> MLNQELELSLNMAFARAREHRHEFMTVEHLLLALLSNPSAREALEACSVDLVALRQELEAFIEQTTPVLPASEEERDTQPTLSFQRVLQRAVFHVQSSGRNEVTGANVLVAIFSEQESQAAYLLRKHEVSRLDVVNFISHGTRKDEPTQSSDPGSQPNSEEQAGGEERTENFTTNLNQLARVGGIDPLIGREKELERAIQVLCRRRKNNPLLVGESGVGKTAIAEGLAWRIVQGDVPEVMADCTIYSLDIGSLLAGTKYRGDFEKRFKALLKQLEQDTNSILFIDEIHTIIGAGAASGGQVDAANLIKPLLSSGKIRVIGSTTYQEFSNIFEKDRALARRFQKIDITEPSIEETVQIINGLKPKYEAHHDVRYTAKAVRAAVELAVKYINDRHLPDKAIDVIDEAGARARLMPVSKRKKTVNVADIESVVARIARIPEKSVSQSDRDTLKNLGDRLKMLVFGQ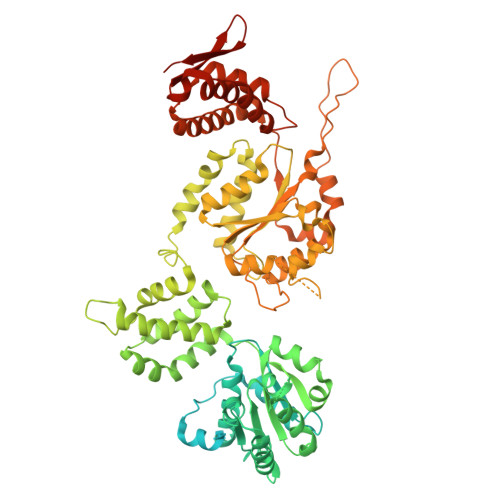DKAIEALTEAIKMARAGLGHEHKPVGSFLFAGPTGVGKTEVTVQLSKALGIELLRFDMSEYMERHTVSRLIGAPPGYVGFDQGGLLTDAVIKHPHAVLLLDEIEKAHPDVFNILLQVMDNGTLTDNNGRKADFRNVVLVMTTNAGVRETERKSIGLIHQDNSTDAMEEIKKIFTPEFRNRLDNIIWFDHLSTDVIHQVVDKFIVELQVQLDQKGVSLEVSQEARNWLAEKGYDRAMGARPMARVIQDNLKKPLANELLFGSLVDGGQVTVALDKEKNELTYGFQSAQKHKAEAAH> TGGK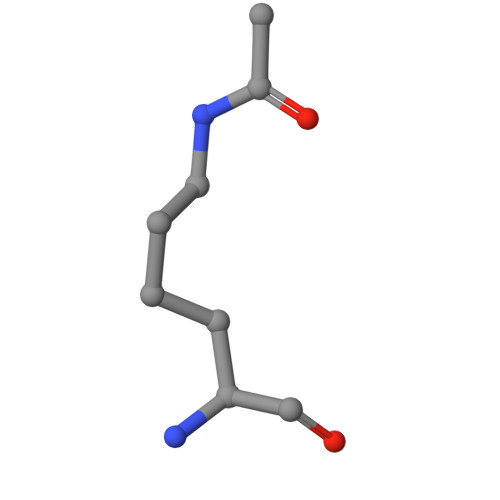APR> GSHMVNIIQDFIPVGANNRPGYAMTPLYITVHNTANTAVGADAAAHARYLK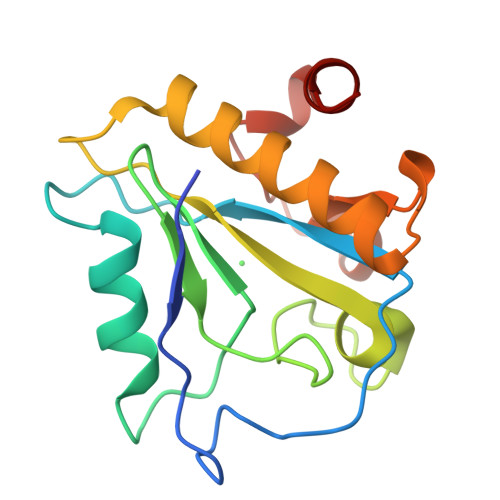NPDTTTSWHFTVDDTEIYQHLPLNENGWHAGDGNGSGNRASIGIEICENADGDFAKATANAQWLIKTLMAEHNISLANVVPHKYWSGKECPRKLLDTWDSFKAGIG>[2x]MVSAGIEAMNVFGGTAYLDVMELAKYRHLDTARFENLLMKEKAVA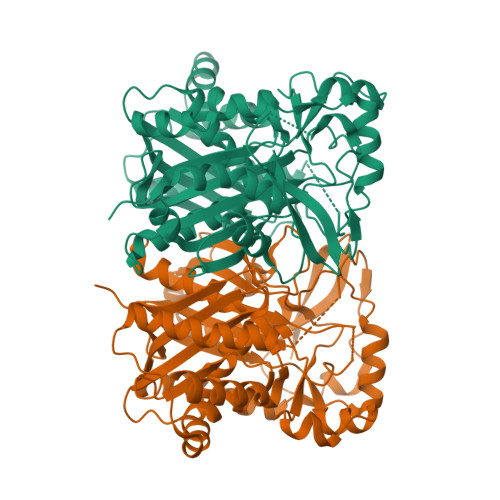LPYEDPVTFGVNAAKPIIDALSEAEKDRIELLITCSESGIDFGKSLSTYIHEYLGLNRNCRLFEVKQAAYSGTAGFQMAVNFILSQTSPGAKALVIASDISRFLIAEGGDALSEDWSYAEPSAGAGAVAVLVGENPEVFQIDPGANGYYGYEVMDTCRPIPDSEAGDSDLSLMSYLDCCEQTFLEYQKRVPGANYQDTFQYLAYHTPFGGMVKGAHRTMMRKVAKVKTSGIETDFLTRVKPGLNYCQRVGNIMGAALFLALASTIDQGRFDTPKRIGCFSYGSGCCSEFYSGITTPQGQERQRTFGIEKHLDRRYQLSMEEYELLFKGSGMVRFGTRNVKLDFEMIPGIMQSTQEKPRLFLEEISEFHRKYRWIS> IESIIKTATDTVKSEINAELGVVPSLNAVETGATSNTEPEEAIQTRTVINQHGVSETLVENFLSRAALVSKRSFEYKDHTSSAAQADKNFFKWTINTRSFVQLRRKLELFTYLRFDAEITILTTVAVNGSGNNTYVGLPDLT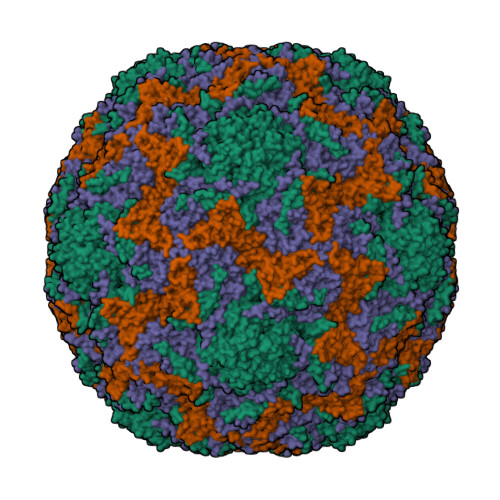LQAMFVPTGALTPEKQDSFHWQSGSNASVFFKISDPPARITIPFMCINSAYSVFYDGFAGFEKNGLYGINPADTIGNLCVRIVNEHQPVGFTVTVRVYMKPKHIKAWAPRPPRTLPYMSIANANYKGKERAPNALNAIIGNRDSVKTMPHNIV;> SPSAEACGYSDRVLQLKLGNSAIVTQEAANYCCAYGEWPNYLPDHEAVAIDKPTQPETATDRFYTLKSVKWETGSTGWWWKLPDALNNIGMFGQNVQHHYLYRSGFLIHVQCNATKFHQGALLVVAIPEHQRGAHNTNTSPGFDDIMKGEEGGTFNHPYVLDDGTSLACATIFPHQWINLRTNNSATIVLPWMNAAPMDFPLRHNQWTLAIIPVVPLGTRTTSSMVPITVSIAPMCCEFNGLRHAITQ;> GVPTYLLPGSGQFLTTDDHSSAPALPCFNPTPEMHIPGQVRNMLEVVQVESMMEINNTESAVGMERLKVDISALTDVDQLLFNIPLDIQLDGPLRNTLVGNISRYYTHWSGSLEMTFMFCGSFMATGKLILCYTPPGGSCPTTRETAMLGTHIVWDFGLQSSVTLIIPWISGSHYRMFNNDAKSTNANVGYVTCFMQTNLIVPSESSDTCSLIGFIAAKDDFSLRLMRDSPDIGQLDHLHAAEAAYQ;> MGAQVTRQQTGTHENANIATNGSHITYNQINFYKDSYAASASKQDFSQDPSKFTEPVVEGLKAGAPVLK4-[[1,1-bis(oxidanylidene)-7-propan-2-yl-4~{H}-1$l^{6},2,4-benzothiadiazin-3-yl]amino]-2,6-bis(chloranyl)phenol | C16 H15 Cl2 N3 O3 S | 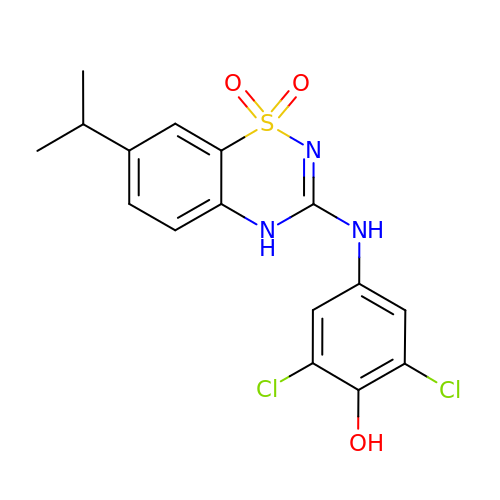MZBADMWUAMNYAJ-UHFFFAOYSA-N2-[(6-AMINO-7H-PURIN-8-YL)THIO]ACETAMIDE 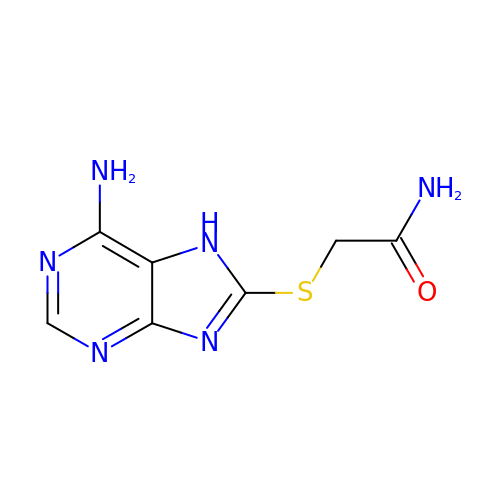| C7 H8 N6 O S | LZGZHYMVMFIEIY-UHFFFAOYSA-N>GAMGSSTQTAEDKEEPLHSIISSTESVQGSTSKHEFQAETKKLLDIVARSLYSEKEVFIRELISNASDALEKLRHKLVSDGQALPEMEIHLQTNAEKGTITIQDTGIGMTQEELVSNLGTIARSGSKAFLDALQNQAEASSKIIGQFGVGFYSAFMVADRVEVYSRSAAPGSLGYQWLSDGSGVFEIAEASGVRTGTKIIIHLKSDCKEFSSEARVRDVVTKYSNFVSFPLYLNGRRMNTLQAIWMMDPKDVREWQHEEFYRYVAQAHDKPRYTLHYKTDAPLNIRSIFYVPDMKPSMFDVSRELGSSVALYSRKVLIQTKATDILPKWLRFIRGVVDSEDIPLNLSRELLQESALIRKLRDVLQQRLIKFFIDQSKKDAEKYAKFFEDYGLFMREG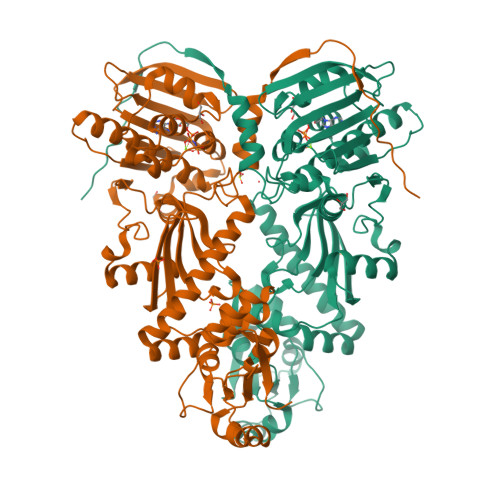IVTATEQEVKEDIAKLLRYESSALPSGQLTSLSEYASRMRAGTRNIYYLCAPNRHLAEHSPYYEAMKKKDTEVLFCFEQFDELTLLHLREFDKKKLISVETDI[2x]>[4x]MPQLHYVPYDTPVEDVMRILKESGTLVIRNFLDQNTVQKVQDEVDDYVRNWNPGPKYNHDIKNVGSKTKQPSNLSLMSKTYRCEVLNHPWMHAICERMFGPTYGDYWFNGGAILHLEPGENTQPIHQDHVFYQISKWRRPTDPDLTINFTMALTEFTVENGGTRVCPGSHLWENGHASPAEEDMVPVLMQPGDALILPGSMWHSAGANRTSEYRRGFATSFHPCHFTPIESHHHLPREMVEEMTPLVQKMLGFRTLNLHNNVKVWKAGEGNLEDATGLKSVAAKLAAALEHHHHHH

Here, we report the biochemical and structural characterizations of the unusually promiscuous and catalytically versatile Fe/αKG oxygenase SptF, involved in the biosynthesis of fungal meroterpenoid emervaridones. The in vitro analysis revealed that SptF catalyzes several continuous oxidation reactions, including hydroxylation, desaturation, epoxidation, and skeletal rearrangement. Fe/αKG oxygenases utilize αKG as a co-substrate and Fe(II) as a cofactor. Through the oxidative decarboxylation of αKG, a reactive Fe(IV)-oxo intermediate is generated to activate a selective aliphatic C–H bond, which is normally difficult to cleave due to high bond-dissociation energy, and then oxidative products are generated following radical recombination.

SptF also catalyzed the formation of cyclopropane-ring-fused, highly congested 5/3/5/5/6/6 and 5/3/6/6/6 cyclic skeletons from structurally distinct meroterpenoid terretonins. Interestingly, the unnatural substrate 15 shows a different ligand binding mode in the active site. The D-ring of 15 forms a hydrogen-bond network with Thr148 and Leu199 via water molecules, but also forms a hydrogen bond directly with Asn150. Notably, the lid-like loop region was not observed upon the binding of 15, while the conformations of the other active site residues were almost identical. In this structure, Phe133 and Ile231 are located close to the methyl groups of C8, C10, and C13, and potentially form hydrophobic interactions. The C6 enol group of 15 is close to the iron with a distance of 3.7 Å, suggesting that the enolic hydrogen atom is abstracted to initiate the cyclopropane-ring formation reaction via the proposed path c in Supplementary Fig. 9. Interestingly, only the N150A variant lacked the activity for the conversion of 15 into 16, suggesting that the direct hydrogen bonding between Asn150 and 15 is crucial for the substrate binding. In contrast, while Ile63 and Asn65 on the lid-like loop region are important for the formation of 4 and 5, these residues are not essential for the reaction with the unnatural substrate 15, suggesting that 15 is mainly recognized by active site residues but not via residues on the lid-like loop. As a result, all the variants still maintained 24–40% and 56–84% activities toward 10 and 13, but dramatically decreased activities toward 21, 24, and 28 (<20%). These observations indicated that the lid-like loop region is crucial for the steroid substrate recognition, but not essential for the meroterpenoid substrates, which is consistent with the absence of the electron density of the loop in the complex structure with 15.> GFKANLSLLRRPGEKTYTQR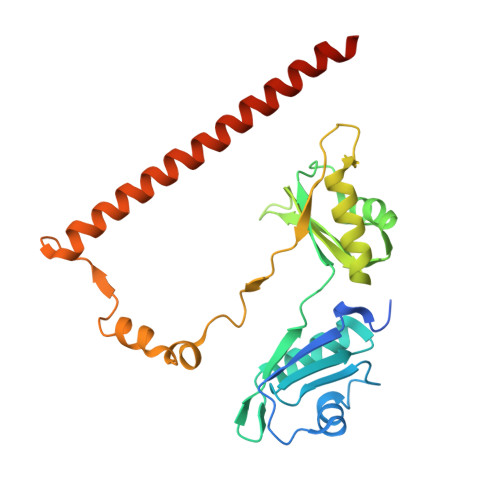CRLFVGNLPADITEDEFKRLFAKYGEPGEVFINKGKGFGFIKLESRALAEIAKAELDDTPMRGRQLRVRFATHAAALSVRNLSPYVSNELLEEAFSQFGPIERAVVIVDDRGRSTGKGIVEFASKPAARKAFERCSEGVFLLTTTPRPVIVEPLEQLDDEDGLPEKLAQKNPMYQKERETPPRFAQHGTFEYEYSQRWKSLDEMEKQQREQVEKNMKDAKDKLESEMEDAYHEHQANLL> MEPPGRRECPFPSWRFPGL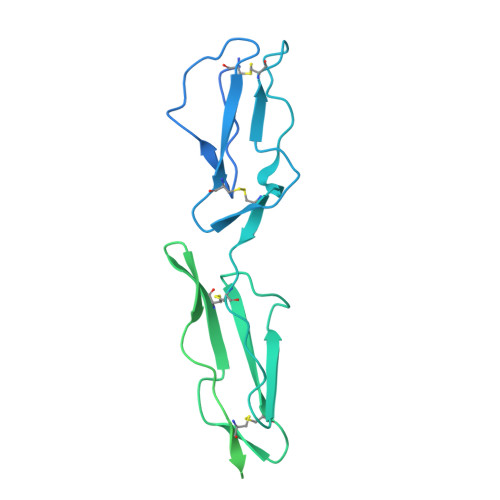LLAAMVLLLYSFSDACEEPPTFEAMELIGKPKPYYEIGERVDYKCKKGYFYIPPLATHTICDRNHTWLPVSDDACYRETCPYIRDPLNGQAVPANGTYEFGYQMHFICNEGYYLIGEEILYCELKGSVAIWSGKPPICEKVLCTPPPKIKNGKHTFSEVEVFEYLDAVTYSCDPAPGPDPFSLIGESTIYCGDNSVWSRAAPECKVVKCRFPVVENGKQISGFGKKFYYKATVMFECDKGFYLDGSDTIVCDSNSTWDPPVPKCLKVLPPSSTKPPALSHSVSTSSTTKSPASSASGPRPTYKPPVSNYPGYPKPEEGILDSLDVWVIAVIVIAIVVGVAVICVVPYRYLQRRKKKGTYLTDETHREVKFTSL PHENANTHRENE 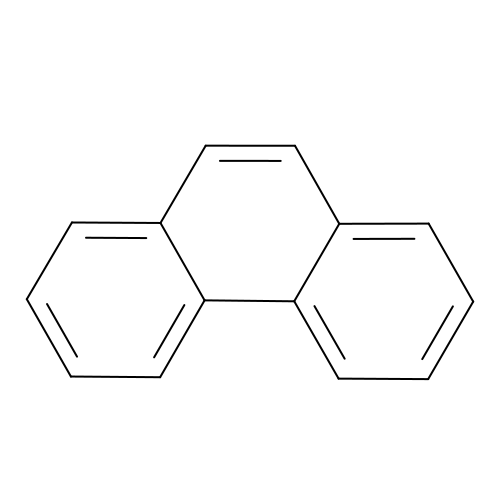| C14 H10 | YNPNZTXNASCQKK-UHFFFAOYSA-N> MGSDKIHHHHHHMKSYRKELWFHTKRRREFINITPLLEECVRESGIKEGLLLCNAMHITASVFINDDEPGLHHDFEVWLEKLAPEKPYSQYKHNDTGEDNADAHLKRTIMGREVVIAITDR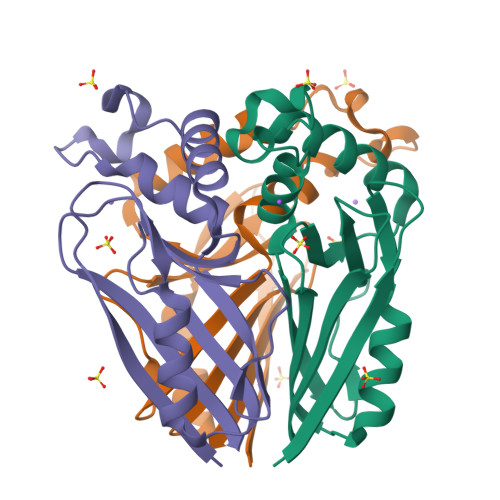KMDLGPWEQVFYGEFDGMRPKRVLVKIIGE> HHHHHHDDDDKRTLPGEGTQVHPRAPLLQILKVAGAQE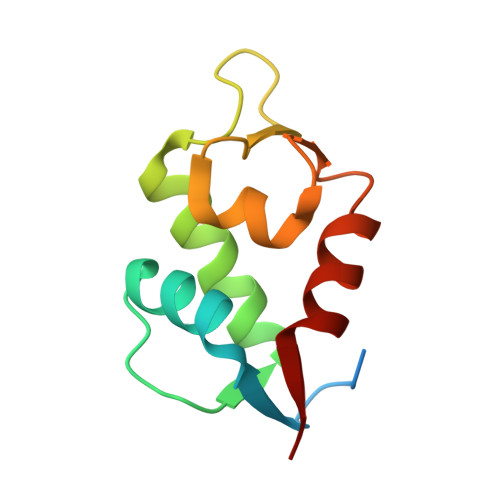EVFTVKEVMHYLGQYIMMKQLYDKQRQHIVHCHDDPLGELLEVGSFSVKNPSPLYEMLKRNLVIL Imidazoleglycerol-Phosphate Dehydratase (IGPD, EC 4.2.1.19) is inhibited by 3-amino-1,2,4-triazole (3AT), as well as the experimental herbicide, (R)-2-hydroxy-3-(1,2,4-triazol-1-yl) propylphosphonate, (R)-C348 and other compounds including β-Carboxamido phosphates and Pyrrole aldehydes. The predicted ORF of Acanthamoeba IGPD gene is 594 nucleotides in length and codes for a putative protein of 197 amino acids with a predicted molecular weight of 21.4 kDa. The conservation of the oligomeric state is critical for positioning the two imperfectly repeated metal binding motifs (D/NXHHXXE) from each subunit on the molecular two-fold axes of the particle, generating the 24 active sites that each contain two octahedrally coordinated manganese (II) ions. The monomer also shares the typical IGPD duplicated fold, with a bundle of 4 α-helices sandwiched between two anti-parallel β-sheets.

We further demonstrate that known inhibitors of IGPD, 3AT and (R)-C348, act to restrict the growth and development of Acanthamoeba and we determine the structure of the complex between Acanthamoeba IGPD and the most potent inhibitor, (R)-C348, to analyse the molecular basis of its potency. Within the active site the inhibitor binds with its N-linked 1,2,4-triazole ring positioned between the two manganese ions, with the N2 and N4 nitrogen atoms residing within the coordination sphere of Mn1 and Mn2, respectively. The C3-OH substituent group of the inhibitor acts as a second non-protein ligand to Mn1, with the sixth ligand position around Mn2 being occupied by a water molecule (HOH1) that has been proposed to have a key role in accepting a proton from the substrate’s imidazole ring during the initial stages of the reaction catalysed by IGPD. The residues from the metal binding motifs complete the coordination of each metal ion; Mn1; H67A’, H40A, H162A and E166A and Mn2; H66A’, E70A’, H138A’, H163A with a Mn-Mn distance of 6.6 Å. The phosphonate group of the inhibitor sits within a predominantly positively charged pocket surrounded by residues from subunits A and C, which include K170A, R92C and R114C, and a water-mediated interaction (HOH5) with H48A. The extensive network of hydrogen bonds surrounding the phosphonate binding site is completed by S191C and K193C from the C-terminal loop of the protein, which occupies a position that essentially shields the active site from the external solvent. In the Ac_IGPD/(R)-C348 complex the conformation of the C-terminal loop and the interactions it makes with the phosphonate group of the inhibitor match those observed in previously determined complexes of Arabidopsis thaliana_IGPD in complex with the substrate IGP, whose mode of binding resembles that of the imidazolate reaction intermediate.

>[12x]MEKREAQVARETGETKIEVRLSLDGTGVSDVKTGIGFLDHMLSALAKHGRFDLYLRCAGDLHVDDHHTSEDCAIVLGQAFRQAIGERKGIKRYGSAYAPLDESLARAVVDISSRPFAVIDLKLKREKIGELSCEMIPHVLHSFATSANLTLHVEVLYGANDHHKAESAFKATALALREAVTKDGPADAVPSTKGVLE nevanimibe | C27 H39 N3 O | 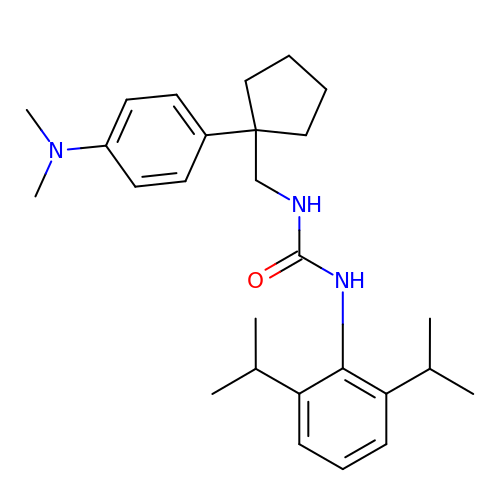PKKNCEXEVUFFFI-UHFFFAOYSA-N> GSREEPSDLEELEQFAKTFKQRRIKLGFTQGDVGLAMGKLYGNDFSQTTISRFEALNLSFKNMCKLKPLLEKWLNDAENLSSDSSLSSPSALNSPGIEGLSRRRKKRTSIETNIRVALEKSFLENQKPTSEEITMIADQLNMEKEVIRVWFCNRRQK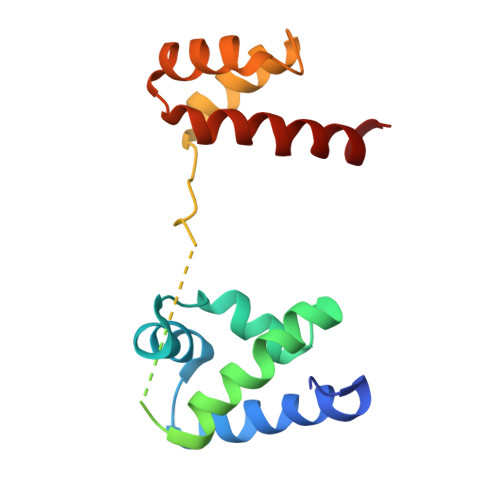EKRINP>ANEVIKCKAAVAWEAGKPLSIEEIEVAPPKAHEVRIKIIATAVCHTDAYTLSGADPEGCFPVILGHLGAGIVESVGEGVTKLKAGDTVIPLYIPQCGECKFCLNPKTNLCQKIRVTQGKGLMPDGTSRFTCKGKTILHYMGTSTFSEYTVVADISVAKIDPLAPLDKVCLLGC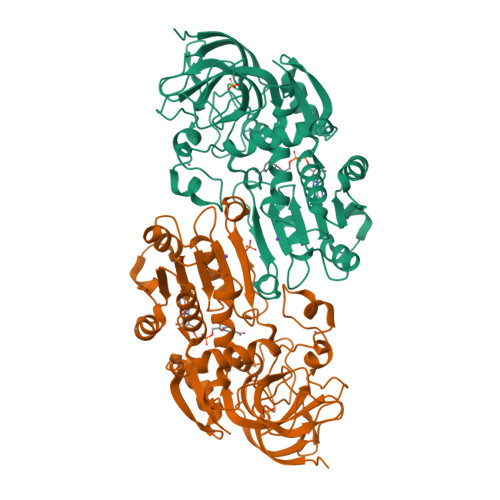GISTGYGAAVNTAKLEPGSVCAVFGLGGVGLAVIMGCKVAGASRIIGVDINKDKFARAKEFGATECINPQDFSKPIQEVLIEMTDGGVDYSFECIGNVKVMRAALEACHKGWGVSVVVGVAASGEEIATRPFQLVTGRTWKGTAFGGWKSVESVPKLVSEYMSKKIKVDEFVTHNLSFDEINKAFELMHSGKSIRTVVKI[2x]(2R,4S,5S)-N-butyl-4-hydroxy-2,7-dimethyl-5-{[N-(4-methylpentanoyl)-L-methionyl]amino}octanamide 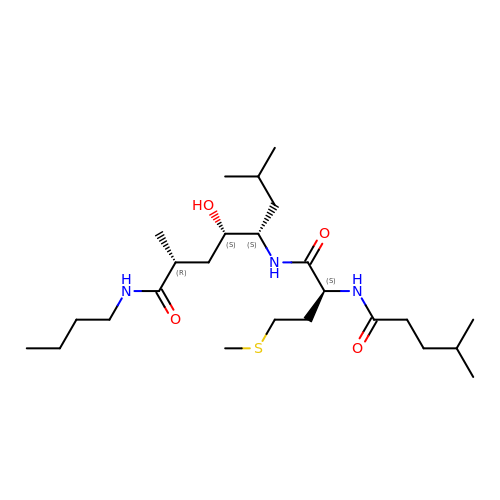| C25 H49 N3 O4 S | XTRMRNMVFXWTCC-MLNNCEHLSA-N> GVDNAEKGKV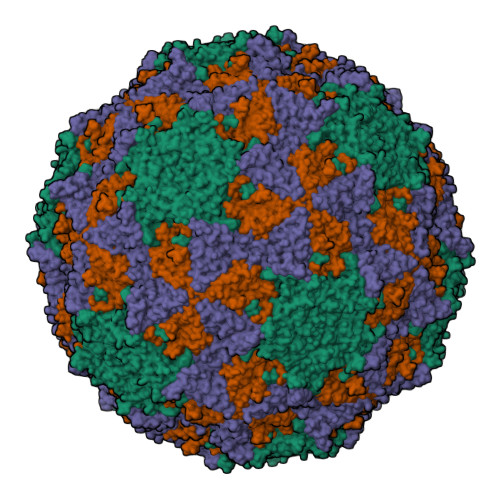SDDNASTDFVAEPVKLPENQTRVSFFYDRSTLSSVLQSTSDVSSKFTPSTAKNLQNSILLTPLPSDIVNNSVLPEQERWISFASPTTQKPPYKTKQDWNFIMFSPFTYYKCDLEVTLSKNDRETISSVVRYVPCGAPSDLSDQTMPQTPSLADTRDPHMWVVGQGTTNQISFVIPYTSPLSVLPSVWFNGFSNFDNSSRFGVAPNADFGRLLLQGQGTFSVHYRYKKMRVFCPRPTVFIPWP;> SPFPVTVREHAGTFFSTTPDTTVPVYGNTISTPFDYMCGEFTDLLSLCKIPTFLGNLDSNKKRIPYFSATNSTPATPLVTYQVTLSCSCMANSMLAAVARNFNQYRGSLNYLFVFTGSAMTKGKFLISYTPPGAGEPKTLDQAMQATYAIWDLGLNSSYNFTVPFISPTHYRQTSYNTPTITSVDGWLTVWQLTPLTYPLGVPNDSHILTLVSGGDDFTLRMPVTFTKYVPQ;> SDRVSSDTAGNTATNTQSTVGRLFGFGQRHKGKHPASCADTATDKVLAAERYYTIKLASWTKTQESFDHIRVPLPHALAGENGGVFSSTLRRHYLCKCGWRIQVQCNASQFHAGSLLVFMAPEFDTSNHSTEVEPRADTAFKVDANWQKHAQILTGHAYVNTTTKVNVPLALNHQNFWQWTTYPHQILNLRTNTTCDLEVPYVNVCPTSSWTQHANWTLVIAVLTPLQYSQGSATTIEITASIQPVKPVFNGLRHTVV;> GNEGVIINNYYSNQYQNSIDLSAN> MQRSTAVVDGSQQVDPAMLAALQSQPSGVTPSDDWAAAMDRILALTTRNPEAFRQQPQANRFSAILEAVVPSRTNPTHEKVLAIVNALTESKAIRKDEAGLIYNALLERVARYNSTNVQANLDRLTTDVREAVAQRERFMHDTNLGSQVALNAFLSTLPANVPRGQEDYVSFISALRLLVAEVPQSEVYQSGPDYFFQTSRQGLQTVNLTQAFKNLQGMWGVRAPVGDRATISSLLTPNTRLLLLLIAPFTNSSTISRDSYLGHLITLYREAIGQTQVDEQTFQEITSVSRALGQQDTGSLEATLNFLLTNRQQKIPSQFTLSTEEERILRYVQQSVSLYLMREGMTPSSALDMTARNMEPSLYSSNRPFINRLMDYLHRAAAMNSEYFTNAILNPHWMPPSGFYTGEFDMPEGDDGFLWDDVSDSIFVPAR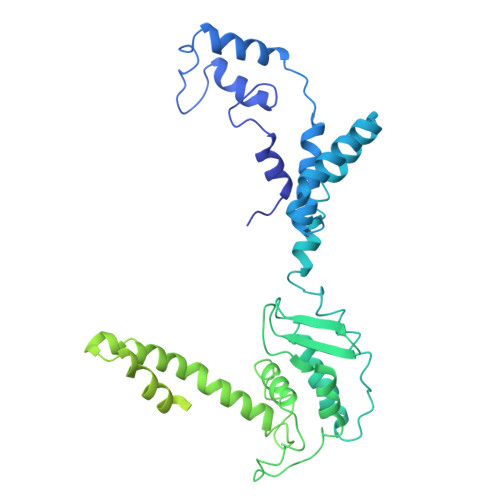YRKKEGGDELPLPLVEAASRGQSPFPSLPSLVSSSNSGRVLRPRLPGETDYLNDPLLQPVRNKNFPNNGVESLVDKMNRWKTYAQEQREWEESQSRPLAGPFSRWRRREDDQDDSADDNSVLDLGGTGASSNPFAHLRPQGRLGRLY> 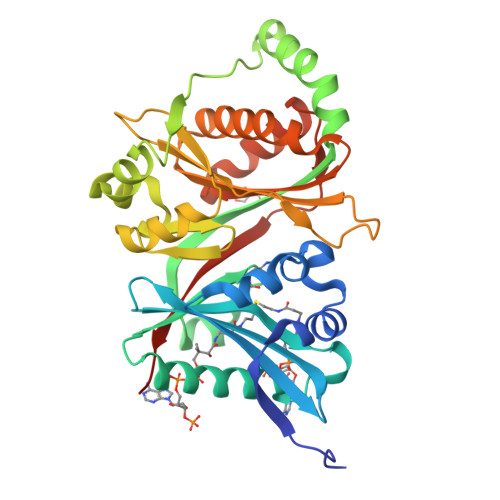MKLEPEAEAEPLDFVVATEREFEEVLAISGGIYGGLDYLPSRYHSWLRDPDRTVVLAKRNGGVIALESVNVIDAGETVLVEGLRVAPWERGKGVAGLLQRFCSQLVKRQHPGVKVARLTRDDQLGPRELKKYRLITKQGILLVRFNASALLAGLGARLAALRTSGTFSPLPTEAVSEAGGDVARLLLSPSVQRDVLPGGTIIQDWQPYRPSESNLRLLAAKGLEWRVDSRARPRVLTLCTRPFPIPHGGDGTWRYLNIDAFGSDGAQVQSQLLWHLQRQAPRLVGLNVMCQLFLEPQLWSQLADFCQVGLGLELVKGYTEQYLLEADIHHHHHH>[4x]MLILKGTKTVDLSKDELTEIIGQFDRVHIDLGTGDGRNIYKLAINDQNTFYIGIDPVKENLFDISKKIIKKPSKGGLSNVVFVIAAAESLPFELKNIADSISILFPWGTLL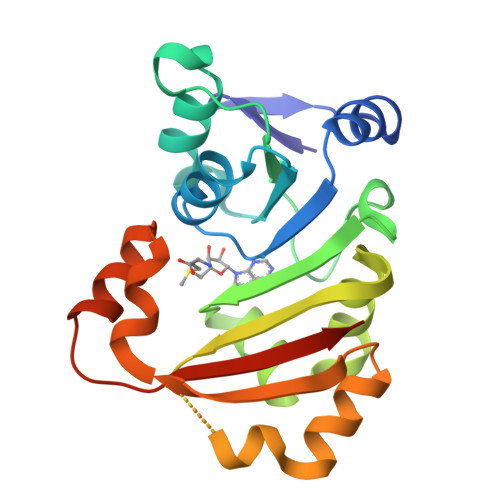EYVIKPNRDILSNVADLAKKEAHFEFVTTYSDSYEEAEIKKRGLPLLSKAYFLSEQYKAELSNSGFRIDDVKELDNEYVKQFNSLWAKRLAFGRKRSFFRVSGHVSKHHHHHHH>MHIPADSFSGASPERKAAVALRSLFTFVAARVVLEQLQGPGGPETTYNQQAYLDLMDFLGTPMKGDGGDEWMAAVMRKNHALALRLMEVREAYLDEFEWGKTMEMASRETREANTRLMRAAAM[4x]

Our data demonstrate that RbcX-II from the green algae C. reinhardtii functions as a bona fide Rubisco assembly chaperone, despite its considerable evolutionary distance from cyanobacterial and eukaryotic RbcX-I proteins. Like all other known RbcX proteins, CrRbcX-IIa is an arc-shaped dimer with a central hydrophobic cleft that binds the C-terminal sequence of the RbcL subunit. Conserved polar residues at the corners of RbcX make critical contacts to the N-domain of an adjacent RbcL, thereby stabilizing the RbcL anti-parallel dimer in a state competent for assembly to the RbcL8 core complex of Rubisco. The green algae Chlamydomonas reinhardtii contains two RbcX-II sequences (CrRbcX-IIa and CrRbcX-IIb, orthologs of AtRbcX-II) and no RbcX-I ortholog.

A stable fragment comprising residues 34–156 lacking the flexible C-terminal 33 residues was produced by subtilisin treatment, as determined by mass spectrometry (MS). We recombinantly expressed and purified the truncated CrRbcX-IIa(34–156) protein for further structural analysis. The structure of the selenomethionine (SeMet)-labeled CrRbcX-IIa(34–156) protein was solved by selenium-single-wavelength anomalous dispersion (Se-SAD) at 2.0 Å resolution. The experimental electron density was readily interpretable. The structural model was built against data to 1.6 Å resolution and refined to final R and Rfree values of 0.177 and 0.206, respectively (see Table 1 for data collection and refinement statistics). The asymmetric unit of the monoclinic unit cell contains four copies of CrRbcX-IIa(34–156) in a two-fold symmetric topology. Each chain consists of a succession of five α-helices. The subunits form arch-shaped, two-fold symmetric dimers with a hydrophobic cleft in the center, similar to other known RbcX structures. The N-terminal sequence of one subunit binds into the central cleft, with residues Met34 and Ile36 reaching into hydrophobic pockets located between the anti-parallel helices α1 and α1’ at the bottom of the cleft. The N-terminal ammonium group of Met34 engages in a tight salt bridge (lengths 2.53 and 2.58 Å) with Asp90 from the opposing dimer, which presumably stabilizes the tetramer arrangement. Indeed, CrRbcX-IIa(34–156) formed mainly tetramers in solution as detected by native-MS.>[5x]SNAMIIRPEQHWFLRLFDWHGSVLSKIIFRLLLNVLMSIIAIISYQWYEQLGIHLTVAPFSLLGIAIAIFLGFRNSASYSRFVEARNLWGTVLIAERTLVRQLRNILPAEHDAHRRIVSYLVAFSWSLKHQLRKTDPTADLRRLLAEERVTEILASSMPTNRILLLAGNEIGQLREAGKLSDITYGLMDNKLDELAHVLGGCERLATTPVPFAYTLILQRTVYLFCTLLPFALVGDLHYMTPFVSVFISYTFLSWDSLAEELEDPFGTAANDLPLNAMCNTIERNLLDMTGQHPLPE

Human bestrophin1 (hBest1) is a Ca2+-activated Cl− channel essential for Cl− transport in retinal pigment epithelium (RPE). Although the structure of hBest1 is still unsolved, two Best1 homolog structures, one from bacteria Klebsiella pneumoniae (KpBest) and the other from chicken (cBest1), have been previously reported. Overall, the channel is a pentameric assembly with a single ion-conducting pathway, which varies in diameter along its length and is constrained at two narrow points: a “neck” contributed by three residues (I62/I66/F70 in KpBest and I76/F80/F84 in hBest1/cBest1) on a transmembrane helix, and an “aperture” formed by a single residue (I180 in KpBest1, I205 in hBest1, and V205 in cBest1) on a cytosolic helix. Here, by electrophysiological and structural analyses, we show that the neck and aperture in hBest1 are both indispensable Ca2+-dependent gates, and their dysregulated opening by rationally designed or patient-derived mutations causes Ca2+-independent leak and elevates Ca2+-dependent channel activity.

Twelve identical residues shared between KpBest and hBest1 on the loop structures within the channel core transmembrane regions were identified as the subjects of alanine substitution, as we reasoned that replacing conserved residues on the (relatively flexible) loops, rather than substitution on the rigid helices, are more likely to be informative without disrupting the overall channel structure. Alanine substitution mutants for each of the 12 residues were generated in KpBest and hBest1 and subjected to crystallography and patch clamp, respectively. All 12 KpBest mutants were purified with a size exclusion profile indistinguishable from the WT, suggesting that the overall integrity of the channel is still retained after alanine substitution. Eleven of the 12 KpBest mutant structures were solved, while 10 of the 12 hBest1 mutants displayed altered channel function.> AILGRSETQECLFFNANWERDRTNQTGVEPCYGDKDKRRHCFATWKNISGSIEIVKQGCWLDDINCYDRTDCIEKKDSPEVYFCCCEGNMCNEKFSYFP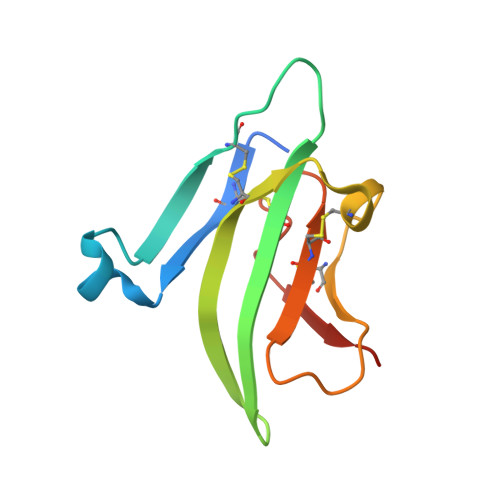EME>[3x]MIQGVIQKIAGPAVIAKGMLGARMYDICKVGEEGLVGEIIRLDGDTAFVQVYEDTSGLKVGEPVVSTGLPLAVELGPGMLNGIYDGIQRPLERIREKTGIYITRGVVVHALDREKKWAWTPMVKPGDEVRGGMVLGTVPEFGFTHKILVPPDVRGRVKEVKPAGEYTVEEPVVVLEDGTELKMYHTWPVRRARPVQRKLDPNTPFLTGMRILDVLFPVAMGGTAAIPGPFGSGKTVTQQSLAKWSNADVVVYVGCGERGNEMTDVLVEFPELTDPKTGGPLMHRTVLIANTSNMPVAAREASIYVGVTIAEYFRDQGFSVALMADSTSRWAEALREISSRLEEMPAEEGYPPYLAARLAAFYERAGKVITLGGEEGAVTIVGAVSPPGGDMSEPVTQSTLRIVGAFWRLDASLAFRRHFPAINWNGSYSLFTSALDPWYRENVAEDYPELRDAISELLQREAGLQEIVQLVGPDALQDAERLVIEVGRIIREDFLQQNAYHEVDAYCSMKKAYGIMKMILAFYKEAEAAIKRGVSIDEILQLPVLERIGRARYVSEEEFPAYFEEAMKEIQGAFKAL;>EYTGITYISGPLLFVENAKDLAYGAIVDIKDGTGRVRGGQVIEVSEEYAVIQVFEETTGLDLATTSVSLVEDVARLGVSKEMLGRRFNGIGKPIDGLPPITPEKRLPITGLPLNPVARRKPEQFIQTGISTIDVMNTLVRGQKLPIFSGSGLPANEIAAQIARQATVRPDLSGEGEKEEPFAVVFAAMGITQRELSYFIQEFERTGALSRSVLFLNKADDPTIERILTPRMALTVAEYLAFEHDYHVLVILTDMTNYCEALREIGAAREEIPGRRGYPGYMYTDLATIYERAGVVEGKKGSVTQIPILSMPDDDRTHPIPDLTGYITEGQIQLSRELHRKGIYPPIDPLPSLSRLMNNGVGKGKTREDHKQVSDQLYSAYANGVDIRKLVAIIGEDALTENDRRYLQFADAFERFFINQGQQNRSIEESLQIAWALLSMLPQGELKRISKDHIGKYY[3x];>KLEAILSQEVEAEIQALLQEAEAKAEAVKREAEEKAKALLQARERALEAQYRAALRRAESAGELLVATARTQARGEVLEEVRRRVREALEALPQKPEWPEVVRKLALEALEALPGAKALVANPEDLPHLEAMARERGVELQAEPALRLGVRAVGAEGKTQVENSLLARMDRAWDAMSSKVAQALWG[2x];>[2x]GMGGLGLIKSLAEKEKQLLERLEAAKKEAEERVKRAEAEAKALLEEAEAKAKALEAQYRERERAETEALLARYRERAEAEAKAVREKAMARLDEAVALVLKEVLP;> SQVSPTRMNLLQRRGQLRLAQKGVDLLKKKRDALVAEFFGLVREAMEARKALDQAAKEAYAALLLAQAFDGPEVVAGAALGVPPLEGVEAEVENVWGSKVPRLKATFPDGALLSPVGTPAYTLEASRAFRRYAEALIRVANTETRLKKIGEEIKKTTRRVNALEQVVIPGIRAQIRFIQQVLEQREREDTFRLKRIKGKIEAREAEEEGG;> MAVIADPETAQGFRLAGLEGYGASSAEEAQSLLETLVERGGYALVAVDEALLPDPERAVERLMRGRDLPVLLPIAGLKEAFQGHDVEGYMRELVRKTIGF;> MADDFAYLNARVRVRRGTLLKESFF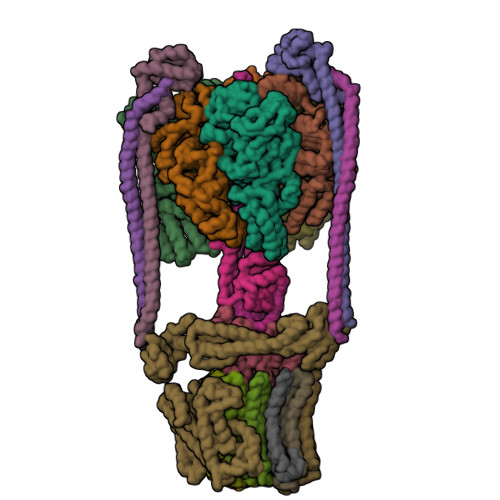QEALDLSFADFLRLLSETVYGGELAGQGLPDVDRAVLRTQAKLVGDLPRLVTGEAREAVRLLLLRNDLHNLQALLRAKATGRPFEEVLLLPGTLREEVWRQAYEAQDPAGMAQVLAVPGHPLARALRAVLRETQDLARVEALLAKRFFEDVAKAAKGLDQPALRDYLALEVDAENLRTAFKLQGSGLAPDAFFLKGGRFVDRVRFARLMEGDYAVLDELSGTPFSGLSGVRDLKALERGLRCVLLKEAKKGVQDPLGVGLVLAYVKEREWEAVRLRLLARRAYFGLPRAQVEEEVVCP;> MIAPMEKLVLAGPKGRAKELLQSLQQAGVVHLETLRPEALSAYQLSPEERAELRRWEAVSAGAEHTLSLLGLEAEPARPFPEGLEAAEKALSPIQAHAEGLTRQKQELEEELALAQAYLEPLERLAALAHGLDKSPFLRVIPFLLTEKELPLVEEALRKALEDRYLLAHEAYAGGVPALVVVHRKEVDQAKAALSRAGVAELRLPGALGELPLSEAARRLKERAEAAPRELSEVRQHLAKLARESASTLQSLWTRAQDEVARLKALEELASGRFGFALLGYVPVKAKPKVEEALARHKENVVYAFEPVDEHHEADRIPVVLDNPPWVKPFELLVSFLNTPKYGTFDPTPVVPIFFPFWFGMIVGDIGYALLFYLVGRWLSGYVKRNEPLVIDLFALKLKPPVLAKLVYILNWMVFWTVVWGLIYGEFFGTFLEHLGVFGTPEHPGLIPILIHRIDTAKTANLLILLSVAFGVVMVFAGLILRAYLGLKHRHMAHFWEGVGYLGGLLGILALAASYLGNLQAGWLSALMYLGFGVFLLSVVMSSIWLMIPEIFTQAGHILSHIRIYAVGAAGGILAGLLTDVGFAMAERLGLIGVLLGIVVAGVLHLLILLLTTLGHMLQPIRLIWVEFFTKFGFYEENGRPYRPFKSVRETQ;>MKKLLVTVLLAVFGALAFAAEEAAASGGLDRGLIAVGMGLAVGLAALGTGVAQARIGAAGVGAIAEDRSNFGTALIFLLLPETLVIFGLLIAFILNGRL[12x]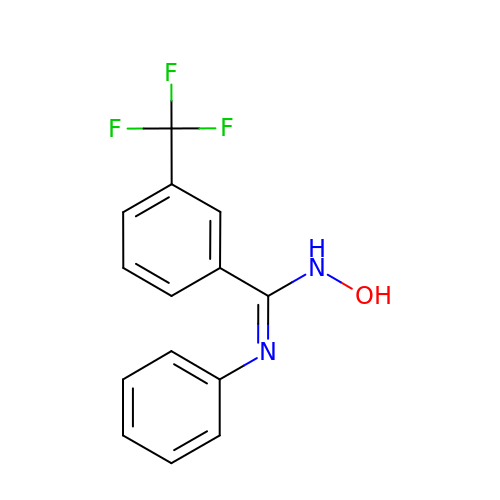N-hydroxy-N'-phenyl-3-(trifluoromethyl)benzenecarboximidamide | C14 H11 F3 N2 O | SFPWZRCGYUTPNJ-UHFFFAOYSA-N> QLVEKLKTQMLDQEELLASTRRDQDNMQAELNRLQAENDASKEEVKEVLQALEELAVNYDQKSQEVEDKTK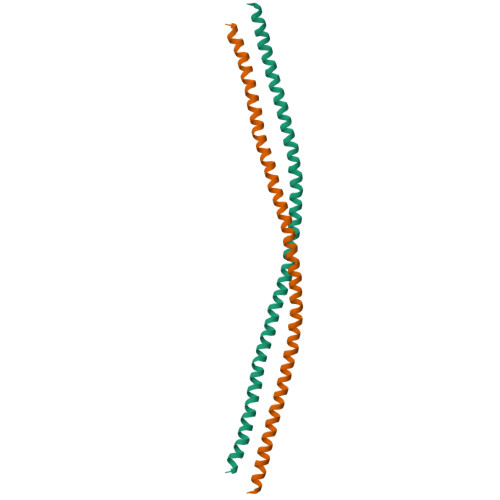EYELLSDELNQKSATLASIDAELQKLKEMTNHQKKRAAEMMASLLKDLAEIG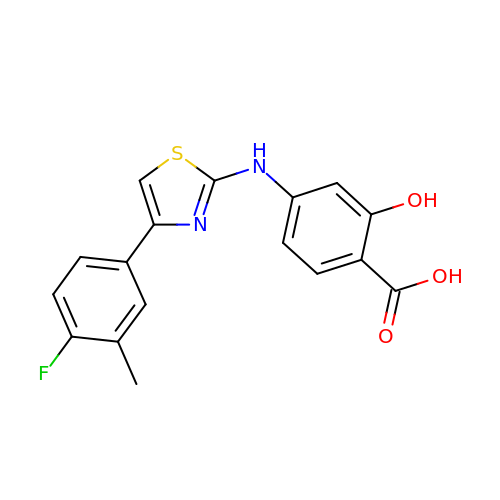4-{[4-(4-fluoro-3-methylphenyl)-1,3-thiazol-2-yl]amino}-2-hydroxybenzoic acid | C17 H13 F N2 O3 S | LKZZDHKJFDTYCH-UHFFFAOYSA-N> SMNEQASGALV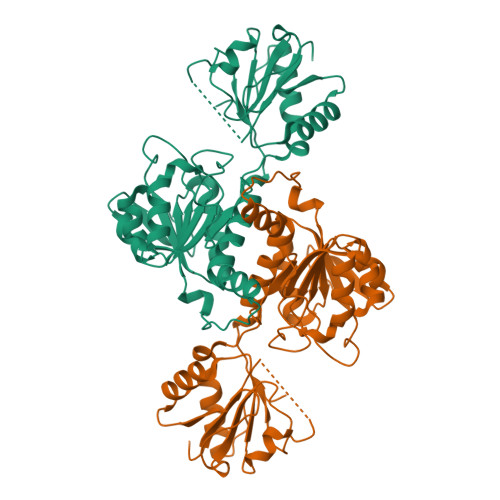FYSAVDIGQDWKSALQAAHPGLDVRIARAGDGHVEGDPEEVRYALVWKPPHGFFARFPNLKLVINLGAGVDALVARDDLPDVPVTRLSDPNMSQMMASFVLFCVLRHARDIPTFERAQREGRWHYVHPRTAAEIRVGVLGLGDLGAAAALELARHGFDVRGWSRTPKALEGVSCFHGLEALPGFLAGSEIVVVMLPLTPETRGLMNAERLAHLPRGAKFINVARGPVVDEAALIAALRSGHIAEATLDVFEVEPLPVGSPLWAMDNVLVTPHLASIAIPRTAAPQIVENIRRIEAGEPVLNQVDPRRGY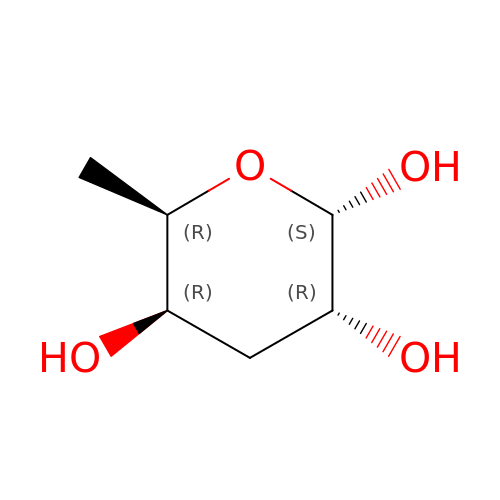alpha-D-Abequopyranose | C6 H12 O4 | KYPWIZMAJMNPMJ-KAZBKCHUSA-N Here, we identify two O-methyltransferases from tea plant: CsFAOMT1 that has a specific O-methyltransferase activity on the 3ʹʹ-position of EGCG to generate EGCG3′′Me, and CsFAOMT2 that predominantly catalyzes the formation of EGCG4″Me. To explain the specificity of CsFAOMT1 and CsFAOMT2, we crystallized both in the presence of EGCG and S-adenosyl-L-homocysteine (SAH), a by-product of the cofactor SAM and determined the structures at a resolution of 2.0 Å for CsFAOMT1 and 2.0 Å for CsFAOMT2. The electron densities for SAH and Mg2+ are unambiguously assigned, but EGCG was not found in either structure. The structural overlap of the monomers of CsFAOMT1 and CsFAOMT2 revealed a root mean square deviation of 0.36 Å over the Cα atom of 190 aligned residues, with the most striking difference occurring in an α-helix (α9) near the substrate binding pocket.

In vitro, enzymatic assays with recombinant CsFAOMT2 protein confirmed that CsFAOMT2 has mainly 4″-O-methyltransferase activity on EGCG and a lower 3″- O-methyltransferase activity. In CsFAOMT1, this α-helix is bent toward the pocket, creating a deep and narrow cleft for substrate binding, whereas in CsFAOMT2 the corresponding α-helix is bent in the opposite direction, resulting in a relatively open and shallow pocket. Two sequence variable residues were identified subsequently: CsFAOMT1-L50 (CsFAOMT2-M50) and CsFAOMT1-Y184 (CsFAOMT2-R184). Consistently, CsFAOMT2-R184Y led to significant increase of 3″-methylation activity and moderate decrease of the ability to methylate the 4″-position of EGCG, and the 3″- and 4″-O-methylation activities of CsFAOMT2-R184Y were decreased by 58% and 54% when M50L mutation was combined in CsFAOMT2, respectively. However, in CsFAOMT2, this residue is mutated to a hydrophobic valine (V49), which makes it possible to accommodate 5″-OMe and leads to the production of dimethyl EGCG. Notably, the side chains of arginine are known to be more flexible than those of tyrosine, meaning that EGCG may bind in a more dynamic manner at the active site of CsFAOMT2 and CsFAOMT1-Y184R mutant, thus conferring them 3″- and 4″-O-methylation activity. The Km values, 95.79 μM for CsFAOMT1 and 20.88 μM for CsFAOMT2, indicated that CsFAOMT2 has a stronger affinity to EGCG than CsFAOMT1. In addition, the kcat/Km value of CsFAOMT2 (6762.45 s−1 M−1) was higher than that of CsFAOMT1 (3830.57 s−1 M−1), suggesting that CsFAOMT2 has higher catalytic efficiency. Additionally, two trace amounts of di-methylated EGCG products (EGCGdi-Me1 and EGCGdi-Me2) were observed in the reaction solution and further validated by LC–MS/MS analysis. Moreover, 3′,5′-dimethyl ether (syringetin) and 3′,4′-dimethyl ether were obtained with myricetin as substrate, which means that CsFAOMT2 could modify myricetin on all the 3′-, 4′-, and 5′-positions of the B ring.

> MADNIVLKTILKSEALQKYIWDTSAYPREHEQLKRLRDATFKKYGDRAVMGVPPDEGLFLSMLLKLMNAKKTLEIGVFTGYSLLTTALALPHDGQIVAIDPNREAFEVGLPCIQKAGVEHKINFIESDAISILNEMLSDEGKLKMEFDFVLVDADKPNYINYHEQAIKLVKVGGVIAYDNTLWRGLVVSKEEEVPERFRANQKPIIELNKHLASDPRVEIAQISIGDGVTLCRRII> MAAKVFESIGKFGLALAVAGGVVNSALYNVDAGHRAVIFDRFRGVQDIVVGEGTHFLIPWVQK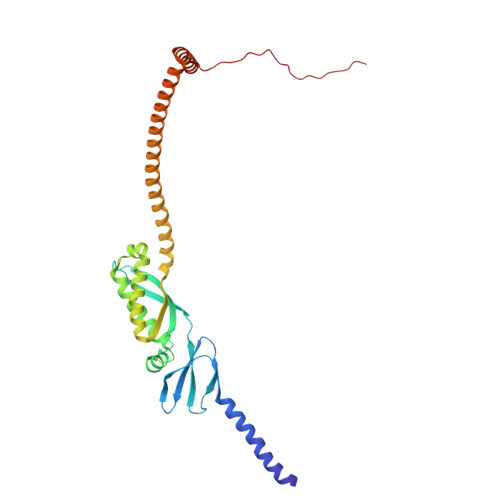PIIFDCRSRPRNVPVITGSKDLQNVNITLRILFRPVASQLPRIFTSIGEDYDERVLPSITTEILKSVVARFDAGELITQRELVSRQVSDDLTERAATFGLILDDVSLTHLTFGKEFTEAVEAKQVAQQEAERARFVVEKAEQQKKAAIISAEGDSKAAELIANSLATAGDGLIELRKLEAAEDIAYQLSRSRNITYLPAGQSVLLQLPQ>[2x]MRGSHHHHHHGSAKNVVLDHDGNLD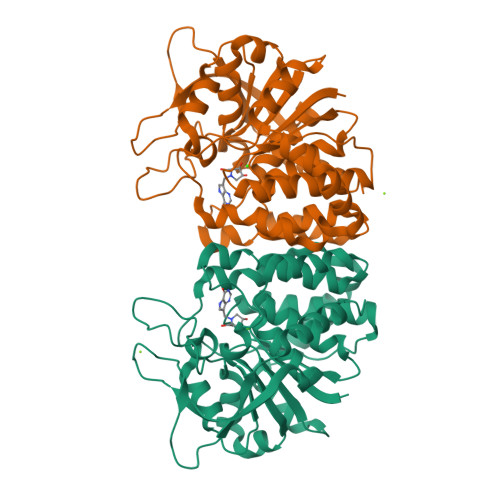DFVAMVLLASNTEKVRLIGALCTDADCFVENGFNVTGKIMCLMHNNMNLPLFPIGKSAATAVNPFPKEWRCLAKNMDDMPILNIPENVELWDKIKAENEKYEGQQLLADLVMNSEEKVTICVTGPLSNVAWCIDKYGEKFTSKVEECVIMGGAVDVRGNVFLPSTDGTAEWNIYWDPASAKTVFGCPGLRRIMFSLDSTNTVPVRSPYVQRFGEQTNFLLSILVGTMWAMCTHCELLRDGDGYYAWDALTAAYVVDQKVANVDPVPIDVVVDKQPNEGATVRTDAENYPLTFVARNPEAEFFLDMLLRSARAC>VNFPNIPAEGVQFRLRARDTGYVIYSRTENPPLVWQYNGPPYDDQLFTLIYGTGPRKNLYAIKSVPNGRVLFSRTSASPYVGNIAGDGTYNDNWFQFIQDDNDPNSFRIYDLASDTVLYSRTTADPKFGNFTGA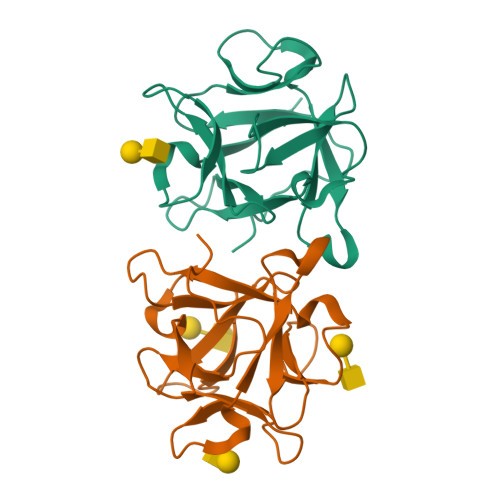KYDDQLWHFELV[4x]> MSRLIFEHQRRLTPPTTRKGTITIEPPPQLPMRTEEVDAERADYLRYLSVVRDNVRAHAAEQRAALEWSHPEPEVLATIPGTRRQWERDPRDRDFLVLRAGRHDVPLDAALKVKDTADEIDLEPVAHSALRGLLDVQRTVRDAPTGLDVAKLARITVIGEADEARAAIRAWIAQAVTWHDPTMLGVALAAPDLESGDWSWLKWLPHVDVPNEADGVGPARYLTTSTAELRERLAPALADRPLFPAESGAALKHLLVVLDDPDADPD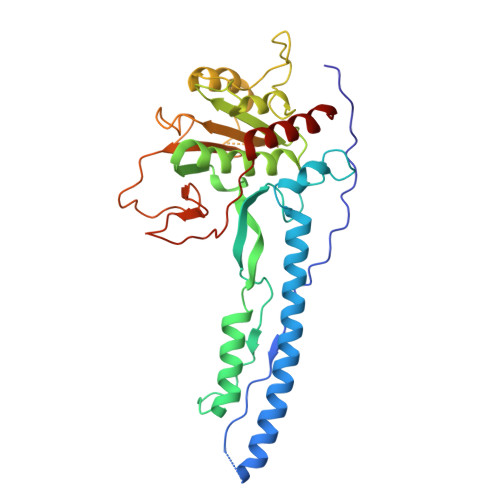DIARKPGLTGVTVIHRTTELPNREQYPDPERPILRVADGRIERWQVGGWQPCVDVADAMSAAEAAHIARRLSRWDSN> MERIWKTGITQHIGHETYIRGYRLLDLVGNLSFAQAIYLILKGELPTERESRMMEAMLVSVIDHGIAPPSAIAARSVASGGNSLNVGVAAGVLAFGSAHGGALEDAMRFIQEGVSSKRSVEDIVKEYLETKKPIPGYGHRYYKDFDPRT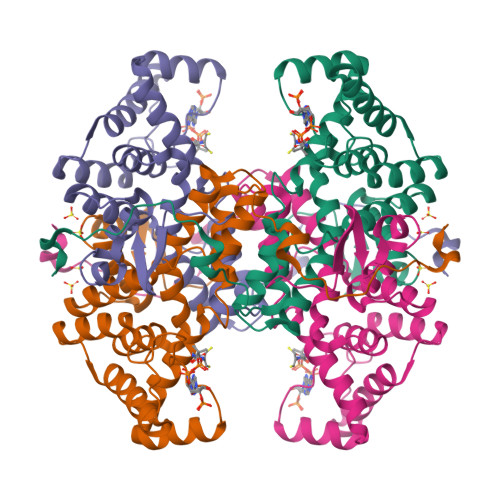KRLMDIARVLEFYGEHCKFAEDVAEEIGRQKGKKLVLNVDGAIAAIASEMGFDWRLGKGFFIIGRVPGLVAHVYEELTTEKPFSKRLDEERDVEYTGSPPRELPQELKKIGGSHHHHHH>[2x]VLAAAPVMVNDCTGKVGQAVAEAAVAAGLRLVPLSLTGPGRGGKRVVIGNVEVDVREVSEREDVVKEVITEYPNVIVVDYTLPAAVNDNAEFYCKQ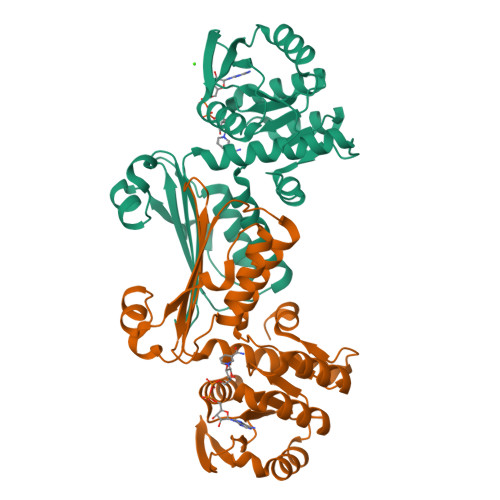GLPFVMGTTGGDREKLLDVARKSGTYSIIAPQMGKQVVAFVAAMEIMAKQFPGAFSGYTLQVTESHQSTKADVSGTALAVISSLRKLGLDFKDEQVELVRDPKEQMTRMGVPEQHLNGHAFHTYKIISPDGTVFFEFKHNVCGRSIYAQGTVDAVLFLSKKIQEKSEKRLYNMIDVLEGGSMR> MAQARKIPLDLPGTRILNGANWANNSATENLATNSGTLIIFDQSTPGQDADRWLIHNYLDGYKIFNMGSNNWASVSRGNTVLGVSEFDGQTCKWSIEYSGNGEEFWIRVPREGGGGAVWTIKPASSQGPTTVFLDLLKETDPNQRIK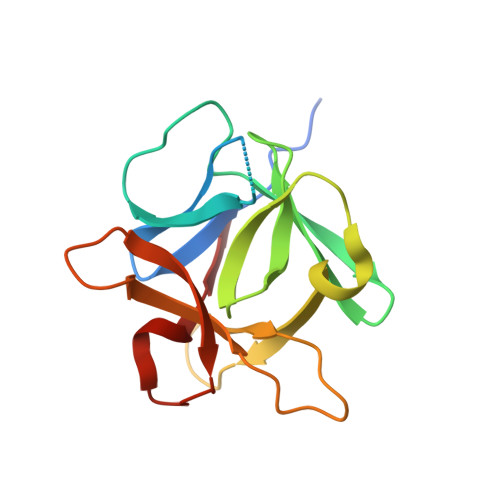FAV>[4x]MVLKTVALVGNPNVGKTTIFNALTGLRQHVGNWPGVTVEKKEGIMEYREKEFLVVDLPGIYSLTAHSIDELIARNFILDGNADVIVDIVDSTCLMRNLFLTLELFEMEVKNIILVLNKFDLLKKKGAKIDIKKMRKELGVPVIPTNAKKGEGVEELKRMIALMAEGKVTTNPIIPRYDEDIEREIKHISELLRGTPLAEKYPIRW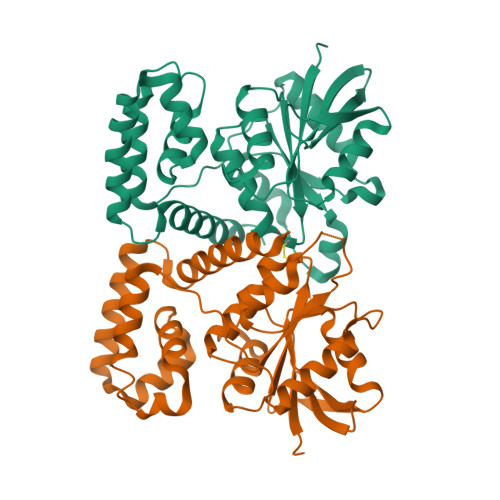LALKLLQRDEEVIKLVLKYLGQEKMDEILKHISELEEKYKRPLDIVIASQKYEFLEQLLRKFVVHE>[8x]KNSLPY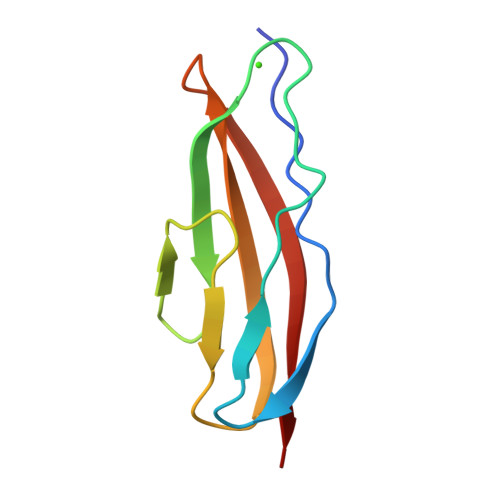GKINGTYKGTEKEKIKFSSEGSFDPDGKIVSYEWDFGDGNKSNEENPEHSYDKVGTYTVKLKVTDDKGESSVSTTTAEIKD N-[(1R,3R)-3-(4-acetylpiperazin-1-yl)cyclohexyl]-4-fluoro-7-methyl-1H-indole-2-carboxamide 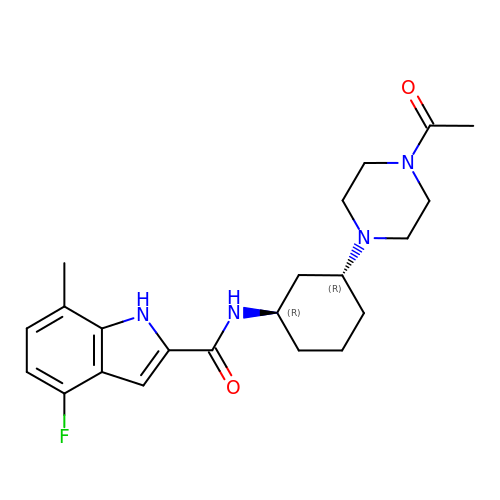| C22 H29 F N4 O2 | PGNLXEBQMQHFNK-IAGOWNOFSA-N> MGSQVKDNKPLVERFETFCLDPSLVTKQANLVHFPPGF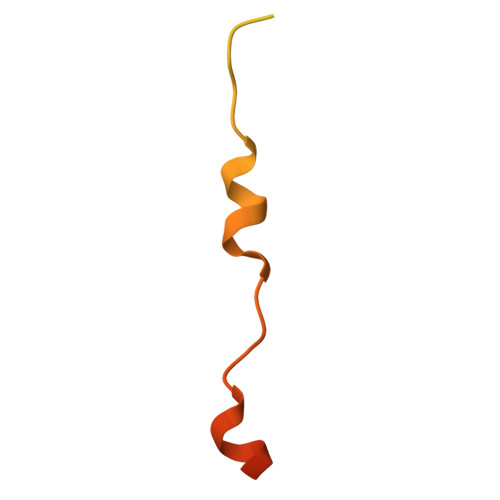QPIPCKPLFFDLALNHVAFPPLEDKLEQKTKSG> MVEYRAEVGQNAYLPCFYTPAAPGNLVPVCWGKGACPVFECGNVVLRTDERDVNYWTSRYWLNGDFRKGDVSLTIENVTLADSGIYCCRIQIPGIMNDEKFNLKLVIK

T-cell immunoglobulin and mucin domain containing protein-3 (TIM-3), also known as Hepatitis A virus cellular receptor 2 (HAVCR2), is involved in regulating innate and adaptive immunity and has thus emerged as a target for numerous therapeutics that are under clinical development. Human (h)TIM-3 consists of a membrane distal variable immunoglobulin (IgV)-like domain involved in ligand interactions, a membrane proximal mucin domain and a transmembrane domain that is connected to an intracellular cytoplasmic tail involved in phosphotyrosine-dependent signaling. Previous structural and biochemical studies have shown that mouse (m)TIM-32 and mTIM-419 bind phosphatidylserine (PtdSer) at the GFCC′ face of the IgV domain in a calcium (Ca++) dependent manner. The IgV-like domain of hTIM-3 has also been demonstrated to bind other ligands such as carcinoembryonic antigen cell adhesion molecule 1 (CEACAM1), high mobility group protein B1 (HMGB1)20 and galectin-91,9,18.

Here we report the high resolution co-crystal structure of hTIM-3 IgV-domain with bound Ca++ that provides a structural basis for understanding hTIM-3 at an atomic level. To do so, we performed the first NMR analysis of a TIM family member and solved a high resolution (1.7 Å). crystal structure of hTIM-3 IgV domain. For example, the AGFCC′C″ and BED face interactions that are important for stabilization of the IgV fold in mTIM-3 including inter-sheet interactions between Trp53 and Val93, a salt bridge between Arg81 and Asp104 and three disulfide bonds were all conserved in hTIM-3. The latter includes disulfide bonds that connect residues Cys38 of the B-C loop and Cys110 of the F strand which provides an anchoring role to stabilize the front and back faces of the hTIM-3 β-sheets and noncanonical disulfide bonds between Cys52 and Cys63, and Cys58 and Cys109. Notably, the B-C loop of mTIM-3 possesses three proline residues (Pro 37, Pro43 and Pro50) whereas hTIM-3 has an additional proline residue at position 45 (Pro37, Pro42, Pro45 and Pro50). Together with the presence of an additional aromatic residue at position 39 (Phe39), the B-C loop (Ala43-Asn47) of hTIM-3 exhibits substantial changes in its conformation signified by its transposition towards (~4 Å) the α–helix connecting the D and E beta strands. In addition, unlike mTIM-3, residues Trp78 and Trp83 of hTIM-3 create a hydrophobic pocket that allows for hydrogen bond formation between the side chain of Thr79 and main chain amide nitrogen of Tyr82. Together, these differences in hTIM-3 result in no apparent outward bending of the C″-D loop in contrast to what is observed in the mTIM-3 structure. Consequently, we observed a different cleft conformation in hTIM-3 compared to mTIM-39, with an extended distance between the C-C′ and F-G loops in mTIM-3 (~11.5 Å) compared to hTIM-3 (~10.0 Å).> GPLGSVLTEAPKVTFKDVAGAEEAKEELKEIVEFLKNPSRFHEMGARIPKGVLLVGPPGVGKTHLARAVAGEARVPFITASGSDFVEMFVGVGAARVRDLFETAKRHAPCIVFIDEIDAVGRKRGSGVGGGNDEREQTLNQLLVEMDGFEKDTAIVVMAATNRPDILDPALLRPGRFDRQIAIDAPDVKGREQILRIHARGKPLAEDVDLALLAKRTPGFVGAD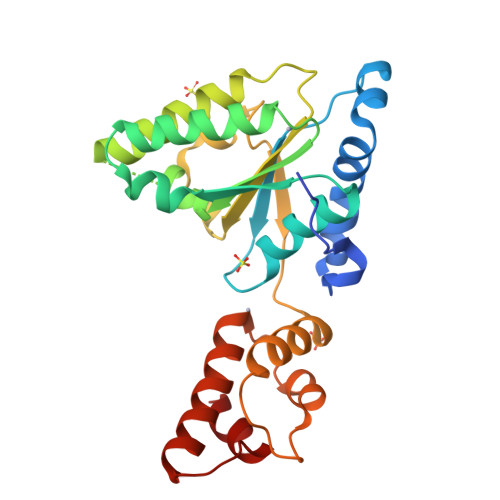LENLLNEAALLAAREGRRKITMKDLEEAAS3-(4-methylpiperazin-1-yl)-5-(pyridin-4-yl)pyridazine | C14 H17 N5 | 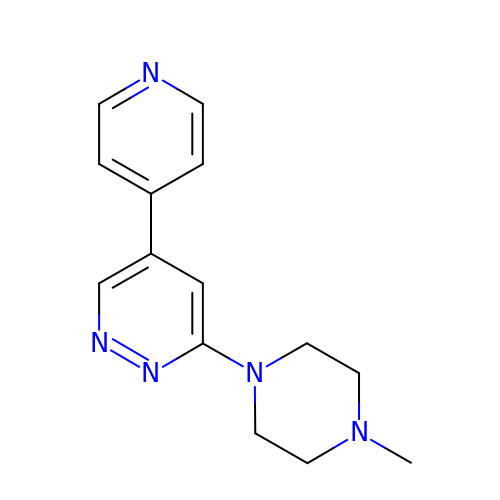ABRBOSKOXBQLEU-UHFFFAOYSA-N(1S,3R,4R,5S)-1,3,4-TRIHYDROXY-5-(3-PHENOXYPROPYL)CYCLOHEXANECARBOXYLIC 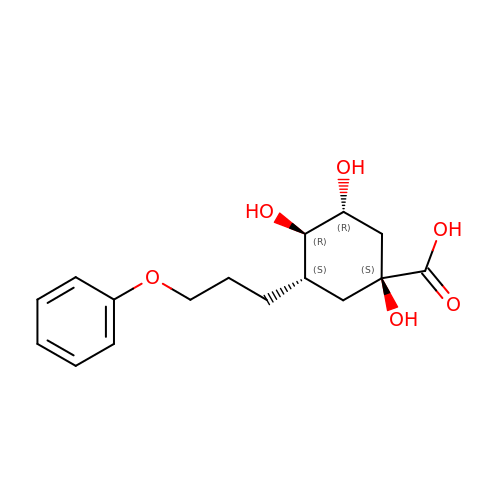ACID | C16 H22 O6 | SCUFESRLGCQXRX-DCDXPUDHSA-N> MAGAKRLELGEALALGSGWRHVCHALLYAPDPGMLFGRIPLRYAILMQMRFDGRLGFPGGFVDTQDRSLEDGLNRELREELGEAAAAFRVERTDYRSSHLTEGPHRVVAHFYAKRLTLEELLAVEAGATRAKDHGLEVLGLVRVPLYTLRDGVGGLP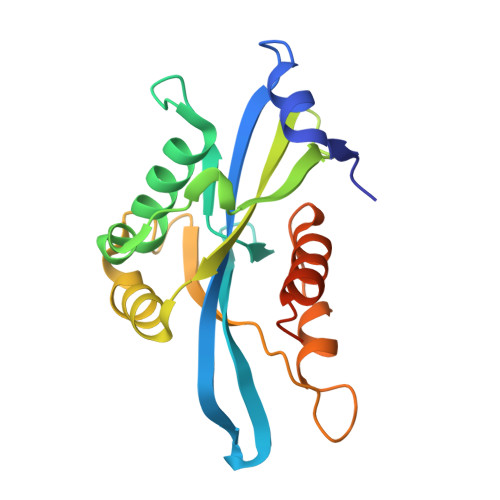TFLENSFIGSAREQLLEALQDLGLLQSGSISGLKIPAHH>MSHHHHHHSMSAAPDSPSSALAALPKDVPNSQPEMVEAVKKHILNMLHLKKRPDVTQPVPKAALLNAIRKLHVGKVGENGYVEIEDDIGRRAEMNELMEQTSEIITFAESGTARKTLHFEISKEGSDLSVVERAEVWLFLK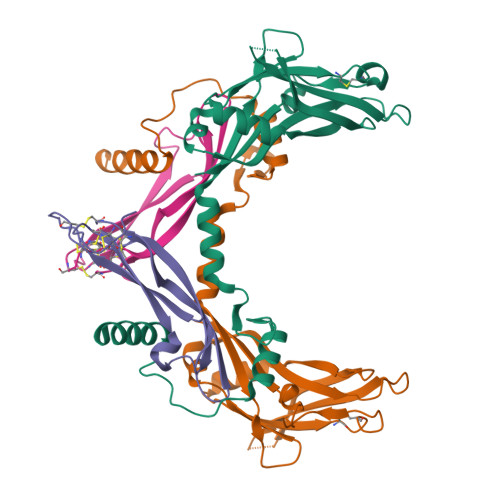VPKANRTRTKVTIRLFQQQKHPQGSLDTGEEAEEVGLKGERSELLLSEKVVDARKSTWHVFPVSSSIQRLLDQGKSSLDVRIACEQCQESGASLVLLGEEKEQSHRPFLMLQARQSEDHPHLEVLFQGP[4x];>[4x]GLECDGKVNICCKKQFFVSFKDIGWNDWIIAPSGYHANYCEGECPSHIAGTSGSSLSFHSTVINHYRMRGHSPFANLKSCCVPTKLRPMSMLYYDDGQNIIKKDIQNMIVEECGCS>[2x]GMKLICSKANLLKGVNIVSKAVPTRTTMAILECILIDASANEIKLMANDMELGIETIIDGTIEERGIIALDAKIFSEIVRKLPDNDVTIETDASFKTVISCEKAKFNIIGKSGDDFSYIPYVERNESIVLSQFTLKEVIRQTIFSIADNDNNKLMTGELFEIEENKLRVVSLDGHRISIRYIEMKNHYDSKKVVVPGKTLQEISKIIPGSADEDVVIYITNNHIVFEFENTTVVSRLIEGEYF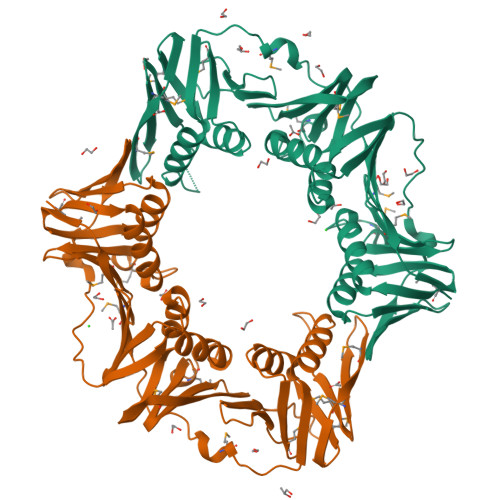KIDQMLSSDYDTKVRINKRELLDCIDRATLLVKEGDKKPIIMNITDGNMELRINSFIGSMNEDIDIDKDGKDIMIGFNPKFFIDALRVIDEEEVNLYMVNPKAPCFIKDDEGKFIYLILPVNFNTAAN Toward this end, we tested sphingomonads for the ability to break the β-aryl ether bond commonly found in lignin and identified and characterized a Nu-class glutathione S-transferase from N. aromaticivorans that acts as a glutathione lyase in the process (NaGSTNu). Here, we find that Nu-class GSTs from N. aromaticivorans (NaGSTNu) and Sphingobium sp. SYK-6 (SYK6GSTNu) can react with both β(R)- and β(S)-GS-HPV in vitro and that NaGSTNu is the sole enzyme required for these reactions in N. aromaticivorans. NaGSTNu is a homodimer; each subunit contains a characteristic N-terminal GST1 (thioredoxin-like) domain (Val39–Gly129),3 a C-terminal GST2 domain (Ser135–Leu257), and N-terminal (Met1–Pro38) and C-terminal (Val258–Phe288) extensions not present in most other characterized classes of GSTs. In addition, this is the first demonstration of a Nu-class GST having a defined physiological role as a glutathione lyase in an organism.

The structures align with each other with an r.m.s. distance of 0.108 Å over 7381 atoms. In NaGSTNu, seven residues make close contacts with GSH1 (Thr51, Asn53, Gln86, Lys99, Ile100, Glu116, and Ser117), and three residues make close contacts with GSH2 (Asn25, Asn53, and Arg177 from the opposite chain in the dimer). In NaGSTNu, a short channel connects the active site to the solvent. The C-terminal Phe288 resides near the active-site channel in one subunit (NaGSTNu closed) and ∼18 Å away from the channel entrance in the other (NaGSTNu open), resulting in a difference between the monomers in the opening to the active-site pocket. The closed NaGSTNu configuration is stabilized by hydrogen bonds between Lys286 and both Lys262 and Arg220. The open configuration lacks these interactions, and its Arg220 side chain has two rotamer positions. For both GS-HPV stereoisomers, there are predicted hydrogen bonds between the γ-hydroxyl and the hydroxyl of Tyr224 and between the HPV phenolic group and the carboxyl group of the C-terminal Phe288.

>SAIAGMSSEYVPPKVWKWDKANGGAFASVNRPVAGPTSERELPVGKHPFQVYSLGTPNGQKATIMLEELLQLGFSEAEYDAWLIKIFEGDQFTSGFVDINPNSKIPAMVDRSGPEPFRVFESGAILMHLAEKFGVFLPTSGPARAECLSWLFWQVGSAPFIGGGFGHFYNYAPIKIEYAIDRYAMETKRLFDVANRRLAESRYLAGDEYTIADLATYTWFGNIYRGEAYGEAATFLSMHEYEHVGRWVGEIDARPGVLRGRLVNSSKGLAERHDASDFDALPPESLQAIVKGF[2x]>GPVLEATMICIDNSEWMRNGDYSPSRLQAQTEAVNLLCGAKTQSNPENTVGILTMAGKGVRVLTTPTSDLGKILACMHGLDVGGEINLTAAIQIAQLALKHRQNKNQRQRIIVFAGSPIKYEKKALEIVGKRLKKNSVSLDIVNFGEDDD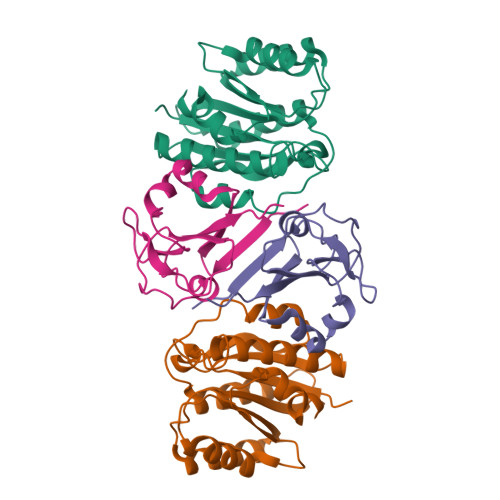EEKPQKLEALLTAVNNNDGSHIVHVPSGANALSDVLLSTPVFTG[2x];>GPAPHEERVGDMRIVNITFSDINSIKNFQPFSQYFDFTLTGPRYNGNIAQFAMIWKIKNPPHNLLGVFFDNNTRDDEDDKYTLEELKQMGNGAKNMYIFWQYEQK[2x]>[4x]MMMIIDCHGHYTVLPKAHDEWREQQKAAFKAGQPAPPYPEISDDEIRETIEANQLRLIKERGADMTIFSPRASAMAPHVGDQSVAVPWAQACNNLIARVVDLFPETFAGVCMLPQSPEADMTSSIAEL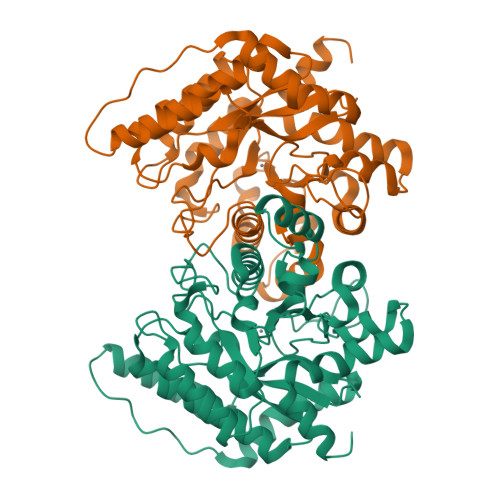ERCVNELGFIGCNLNPDPGGGHFKHPPLTDRFWYPFYEKMVELDVPAMIHVSGSCNPAMHATGAYYLAADTIAFMQLLQGNLFADFPTLRFIIPHGGGAVPYHWGRFRGLADMLKQPSLDTLLMNNVFFDTCVYHQPGINLLADVIDNKNILFGSEMVGAVRGIDPTTGHYFDDTKRYIDALDISDQERHAIFEGNTRRVFPRLDAKLKARGL> GSHHHHHHSIETDRVSKEFIEFLKTFHKTGQEIYKQTKLFLEGMHYKRDLSIEEQSECAQDFYHNVAERMQTRGKVPPERVEKIMDQIEKYIMTRLYKYVFCPETTDDEKKDLAIQKRIRALRWVTPQMLCVPVNEDIPEVSDMVVKAITDIIEMDSKRVPRDKLACITKCSKHIFNAIKITKNEPASADDFLPTLIYIVLKGNPPRLQSNIQYITRFCNPSRLMTGEDGYYFTNLCCAVAFIEKLD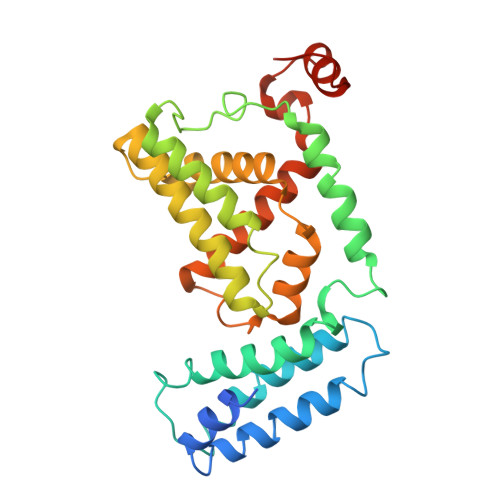AQSLNLSQEDFDRYMSGQTSPRKQEAE> SMDNLLRHLKISKEQITPVVLVVGDPGRVDKIKVVCDSYVDLAYNREYKSVECHYKGQKFLCVSHGVGSAGCAVCFEELCQNGAKVIIRAGSCGSLQPDLIKRGDICICNAAVREDRVSHLLIHGDFPAVGDFDVYDTLNKCAQELN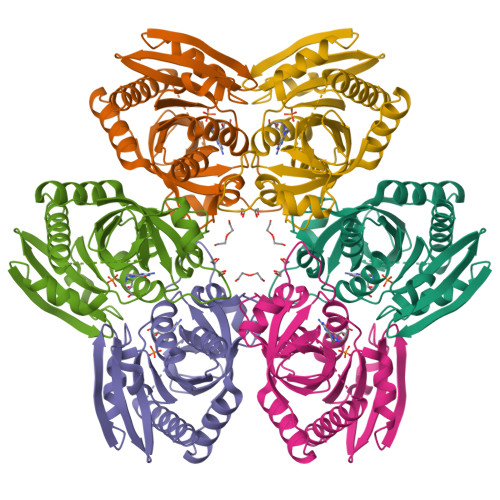VPVFNGISVSSDMYYPNKIIPSRLEDYSKANAAVDEMELATLMVIGTLRKVKTGGILIVDGCPFKWDEGDFDNNLVPHQLENMIKIALGACAKLATKYA>ADRGTETVPGLGQRKQQILNSGGGVWDLAIAMLETKNLGTDYVYGDGKTYDSANFGIFKQNWFMLRTSTSQFKGQTTNQWNNGAVLNSNLQQDIKARQESQNYYGPDKWFAGHRNGESGLSNPYTQDITNYKDAVNWIHDQLASDPKYLSDDTRFWVDVT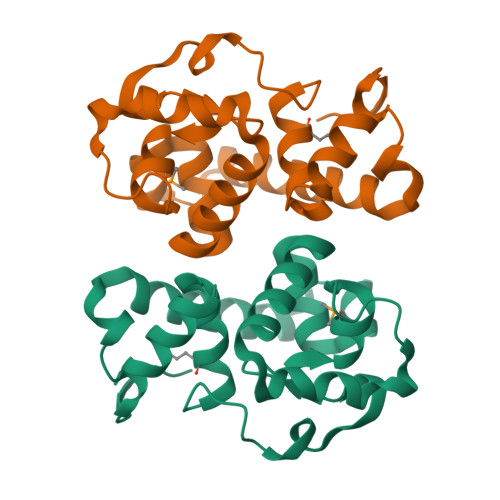AI[2x]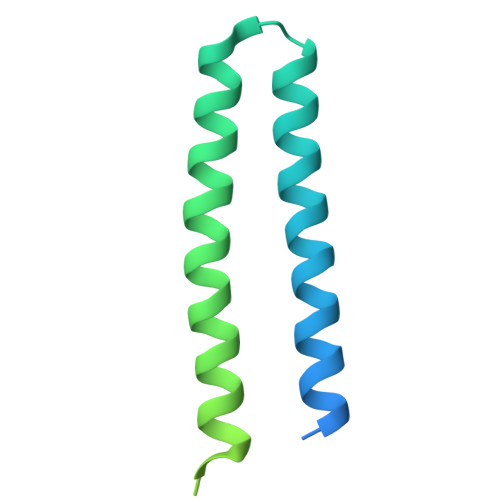> AVSRLLLPSRVRHSYTGKMGAVFIFVGALTVLFGAIAYGEVTAAAATGDAAAVQEAAVSAILGLIILLGINLGLVAATLGGDTAASLSTLAAKASRMGDGDLDVELETRREDEIGDLYAAFDEMRQSVRTSLEDAKNAREDAEQAQKRAEEINTNSHHHHHHH>HHHHHHGSWTSAAVVT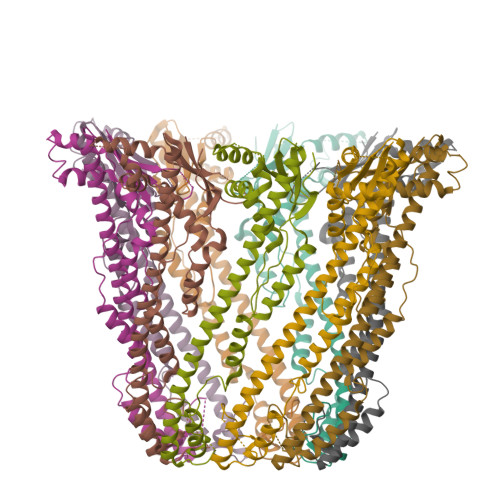PPEPVQWQELEKTFTKLRVLDLDIKIDRTEAFNLFIKKFQSVSLLEEYLRSSPYVMDQLKEAKIDELDLHRAIVALSEKMKAVDDNASKKKDEPSLYTSWTLSFTAPTSEEAQTVLSGYIDYISALVVKESIENVRNKLEIKTQFEKEKLAQDRIKMKNQLDANIQRLNYSLDIANAAGIKKPVYGSGDDPDFSISLGADGIERKLEIEKAVTDVAELNGELRNRQYLVEQLTKANINDVNFTPFKYQLSPSLPV[9x]>AQYEDGKQYTTLEKPVAGAPQVLEFFSFFCPHCYQFEEVLHISDNVKKKLPEGVKMTKYHVNFMGGDLGKDLTQAWAVAMALGVEDKVTVPLFEGVQKTQTIRSASDIRDVFINAGIKGEEYDAAWNSFVVKSLVAQQEKAAADVQLRGVPAMFVNGKYQLNPQGMDTSNMDVFVQQY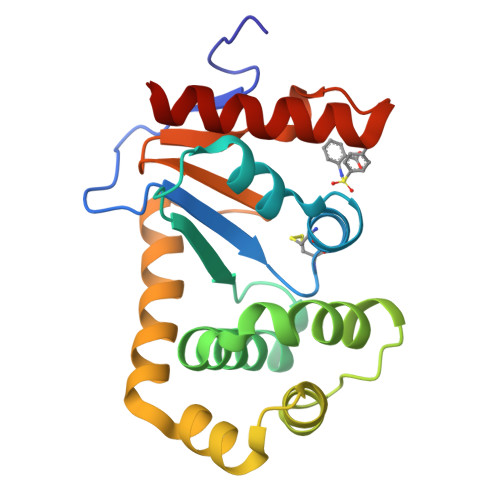ADTVKYLSEK[2x]> MTGSTSHITILTLNINGLNSAIKRHRLASWIKSQDPSVCCIQETHLTCRDTHRLKIKGWRKIYQANGKQKKAGVAILVSDKTDFKPTKIKRDKEGHYIMVKGSIQQEELTILNIYAPNTGAPRFIKQVLSDLQRDLDSHTLIMGDFNTPLSTLDRSTRQKVNKDTQELNSALHQADLIDIYRTLHPKSTEYTFFSAPHHTYSKIDHIVGSKALLSKCKRTEIITNYLSDHSAIKLELRI

The long interspersed nuclear element-1 (LINE-1 or L1) retrotransposon is the only active autonomously replicating retrotransposon in the human genome. To insert a new copy into the genome, L1 uses target-primed reverse transcription (TPRT). The EN initiates this pathway by creating a single-stranded nick in genomic DNA at the semi-specific 5′-TTTT*A-3′ consensus sequence, with the asterisk marking the location of the cleaved phosphodiester bond. Therefore, the EN plays a key role in beginning the process of creating and integrating a new L1 copy into the genome.

To aid our docking efforts, we solved two EN structures by x-ray crystallography. Third, we used additional approaches incorporating structural information to better inform our docking strategies. We used ZINCPharmer to generate the pharmacophore and filter the ZINC database for compounds that matched the pharmacophore, followed by docking with LeDock and AutoDock Vina. The inhibitors identified in this manner were AD28, AD29, AD34, and AD36 (Group 3). In this approach, we screened analogs of this fragment using structural similarity and substructure searches. This provided a series of compounds with minor modifications to the fragment, while others were expanded into larger compounds more likely to inhibit activity. To choose compounds to test in vitro we used template docking with FitDock49, in which analogs were overlaid with the fragment’s location in the EN active site to serve as the initial location from which the docking calculations were completed. The inhibitors chosen from this group were AD41, AD43, and AD50 (Group 4).E. coli aspartate aminotransferase (AAT) is a pyridoxal phosphate (PLP)-dependent enzyme that catalyses the reversible transamination of l-aspartate with α-ketoglutarate, yielding oxaloacetate and l-glutamate. During its catalytic cycle, AAT undergoes hinge movement to switch between an open conformation, in the ligand-free form, and a closed conformation upon association with substrates or inhibitors. Using our approach, we enrich the less populated but catalytically active closed conformation in order to increase catalytic efficiency (kcat/KM) with the non-native substrate l-phenylalanine, leading to altered substrate selectivity. Steady-state kinetics reveal kcat/KM increases of up to 100-fold towards this aromatic amino acid, resulting in a selectivity switch of up to 1900-fold, and structural analyses by room-temperature X-ray crystallography and multitemperature nuclear magnetic resonance (NMR) spectroscopy confirm that the conformational landscape is remodeled to favor the target state.

For example, the VFIT mutant from the Closed Library contains Val, Phe, Ile, and Thr residues at positions 35, 37, 43, and 64, respectively. To determine if these differences in the temperature dependence of exchange could be observed in the crystal state, we also solved the maleate-free structures of WT, HEX, and VFIT at 303 K, and calculated isomorphous difference density maps by subtracting electron density at 278 K. Comparing VFIT data obtained at 278 K and 303 K results in substantial difference density throughout chain A, the chain that opens when WT crystals are soaked to remove maleate. By contrast, similar comparisons for WT and HEX showed relatively little difference density. This analysis confirms that VFIT undergoes larger local conformational changes than either HEX or WT when the temperature of the crystal is increased to 303 K, in agreement with our van’t Hoff analysis of NMR data. The agreement between temperature-dependent X-ray crystallography and NMR data provides strong evidence that the conformational exchange detected in the NMR experiments reflects a dynamic equilibrium between closed and open conformations, with mutations that favor the closed conformation also increasing selectivity toward l-phenylalanine. The relative intensity of the two peaks showed similar temperature dependence, with an increase in the relative intensity of the WT-like peak as temperature was increased to 308 K. Peak deconvolution and integration were used to evaluate the population of the two states, and confirmed that at low temperatures both VFIT and VFIY favor the state resembling that adopted by the closed HEX mutant (T < 288 K or 283 K, respectively). However, unlike HEX, at higher temperatures the alternate conformation with the WT-like peak becomes the favored state.

>[2x]MAHHHHHHVGTFENITAAPADPILGLADLFRADERPGKINLGIGVYFDETGKIPVLTSVKKAEQYLLENETTKTYLGIDGIPEFGRCTQELLFGKGSALINDKRARTAQTPGGTGALRVAADFLAKNTSVKRVWVSNPSWPNHKSVFNSAGLEVREYAYYDAENHTLDFDALINSLNEAQAGDVVLFHGCCHNPTGIDPTLEQWQTLAQLSVEKGWLPLFDFAYQGFARGLEEDAEGLRAFAAMHKELIVASSYSKNFGLYNERVGACTLVAADSETVDRAFSQMKAAIRANYSNPPAHGASVVATILSNDALRAIWEQELTDMRQRIQRMRQLFVNTLQEKGANRDFSFIIKQNGMFSFSGLTKEQVLRLREEFGVYAVASGRVNVAGMTPDNMAPLCEAIVAVL Two of the six classes of the United States Food and Drug Administration (FDA) approved drugs for HIV-1 treatment target the reverse transcriptase (RT) protein, an enzyme critical for the replication cycle of HIV-1. While NNRTIs are allosteric inhibitors that alter the chemical catalysis rate limiting step through conformational changes, NRTIs mimic nucleotides that bind to the active site of RT. Since NRTIs lack the 3′-hydroxyl group necessary for chain elongation, their incorporation results in termination of the viral DNA transcription. In this study, we describe the crystal structures of RT in post-catalytic complexes with double stranded DNA (dsDNA) and two NRTIs —the triphosphate form of cytidine analogue (-)FTC (2′,3′-dideoxy-5-fluoro-3′-thiacytidine) and the triphosphate form of the thymidine analogue d4T (2′,3′-didehydro-2′,3′-dideoxythymidine).

The post-catalytic complex of (-)FTC monophosphate ((-)FTC-MP) incorporated into DNA primer of a dsDNA bound to RT, extends our earlier structural findings with the pre-catalytic complex. The overall structure of the post-catalytic complex of RT together with (-)FTC incorporated in the DNA primer does not highlight any significant changes compared to other structures of RT in complex with dsDNA and NRTIs. The Fo–Fc difference electron density in the N site reveals a double conformation of the incorporated (-)FTC-MP inhibitor. Copy A of (-)FTC-MP was refined to an occupancy of 40% and copy B of (-)FTC-MP was refined to an occupancy of 60%. The cytosine base moieties of both (-)FTC-MP copies maintain only two hydrogen bonds of the classical Watson–Crick base pair with 5-deoxyguanosine (5-dG) in the DNA template. The α-phosphate groups of both copies are in hydrogen bond distance only with the side chain of residue D185. The copy A of (-)FTC-MP establishes further interactions, its primary amino group is in a long distance hydrogen bond (3.4 Å) with a water molecule, and its oxygen of the oxathiolane ring is interacting with the side chain of residue R72 (3.4 Å). No electron density of any Mg+2 ion is observed. Moreover, the absence of electron density for Mg2+ ions indicates that (-)FTC is less susceptible to excision mechanism. The RT post-catalytic complex with (-)FTC-MP evidenced that the 3′-OH of the preceding nucleotide is attacking the α-phosphate, validating our hypothesis that (-)FTC needs to undergo conformational changes in order to get successfully incorporated by RT.

> PISPIETVPVKLKPGMDGPKVKQWPLTEEKIKALVEICTEMEKEGKISKIGPENPYNTPVFAIKKKDSTKWRKLVDFRELNKRTQDFWEVQLGIPHPAGLKKKKSVTVLDVGDAYFSVPLDEDFRKYTAFTIPSINNETPGIRYQYNVLPQGWKGSPAIFQSSMTKILEPFRKQNPDIVIYQYMDDLYVGSDLEIGQHRTKIEELRQHLLRWGLTTPDKKHQKEPPFLWMGYELHPDKWTVQPIVLPEKDSWTVNDICKLVGKLNWASQIYPGIKVRQLSKLLRGTKALTEVIPLTEEAELELAENREILKEPVHGVYYDPSKDLIAEIQKQGQGQWTYQIYQEPFKNLKTGKYARMRGAHTNDVKQLTEAVQKITTESIVIWGKTPKFKLPIQKETWETWWTEYWQATWIPEWEFVNTPPLVKLWYQLEKEPIVGAETFYVDGAANRETKLGKAGYVTNRGRQKVVTLTDTTNQKTELQAIYLALQDSGLEVNIVTDSQYALGIIQAQPDQSESELVNQIIEQLIKKEKVYLAWVPAHKGIGGNEQVDKLVSAGIRKVL;> MGSSHHHHHHSSPISPIETVPVKLKPGMDGPKVKQWPLTEEKIKALVEICTEMEKEGKISKIGPENPYNTPVFAIKKKDSTKWRKLVDFRELNKRTQDFWEVQLGIPHPAGLKKKKSVTVLDVGDAYFSVPLDEDFRKYTAFTIPSINNETPGIRYQYNVLPQGWKGSPAIFQSSMTKILEPFRKQNPDIVIYQYMDDLYVGSDLEIGQHRTKIEELRQHLLRWGLTTPDKKHQKEPPFLWMGYELHPDKWTVQPIVLPEKDSWTVNDIQKLVGKLNWASQIYPGIKVRQLSKLLRGTKALTEVIPLTEEAELELAENREILKEPVHGVYYDPSKDLIAEIQKQGQGQWTYQIYQEPFKNLKTGKYARMRGAHTNDVKQLTEAVQKITTESIVIWGKTPKFKLPIQKETWETWWTEYWQATWIPEWEFVNTPPLVKLWYQLEKEPIVGAETF> GTCCTACCTGGCAGGACGACT;> ACACCGATCACCTGCCACCGTGTCTA;> TCTGATGTGGTAGG;> ACAGTCGTGG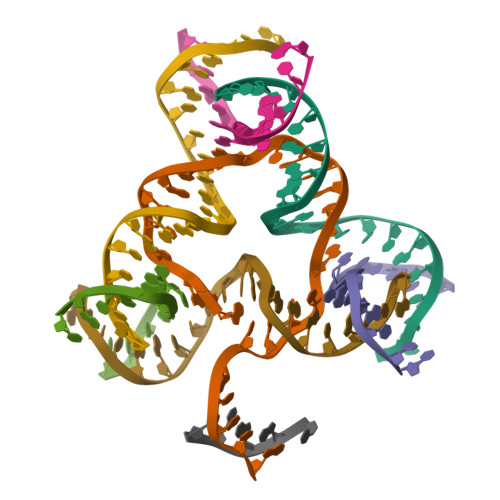TATC;> TGCGTAGTGGTCGC;> CAGATACCTGATCGGACTACG;> GAGCGACCTGTACGGACATCA;> TAGAC> MKILVTGGAGFIGRWVVKRLLQDKHEVWILDNLANSTTANITEFAHDLNLKQCIQGDIKDKKLVAQLFENNSFDLCYHLAASINVQDSIDDARATFENDTIGTFNLLEQCLNYDVKMVFMSTCMVYDKATNIQGISELDPIKPASPYAGSKIAAENMVLSYYYAYKLPVVVIRPFNTYGPFQKTGGEGGVVAI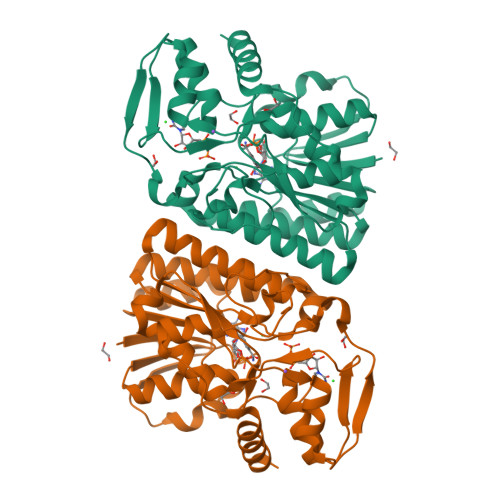FINNKLDNVPLNIYGDGKQTRDLLYVEDCADFVVAAGYSAKANGHIINAGTGQDISINKLAELISGNKVSIQHVTHIHPQSEIQKLLCNYEKAKTILNWEPKVSLEDGVIKTEEWIKSLKINPKEKELEHHHHHH>MDFKENPNLRDNWTDAEGYYRVNIGEVLDKRYNVYGYTGQGVFSNVVRARDNARANQEVAVKIIRNNELMQKTGLKELEFLKKLNDADPDDKFHCLRLFRHFYHKQHLCLVFEPLSMNLREVLKKYGKDVGLHIKAVRSYSQQLFL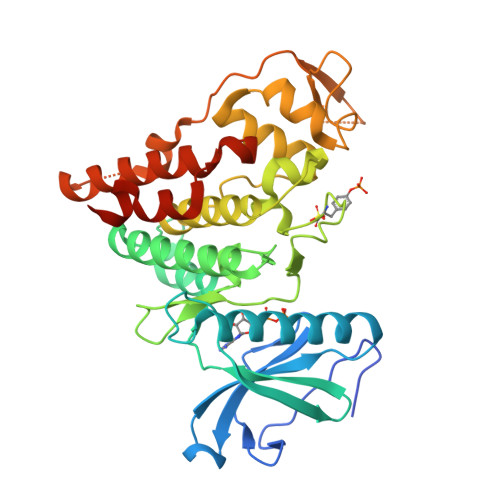ALKLLKRCNILHADIKPDNILVNESKTILKLCDFGSASHVADNDITPYLVSRFYRAPEIIIGKSYDYGIDMWSVGCTLYELYTGKILFPGKTNNHMLKLAMDLKGKMPNKMIRKGVFKDQHFDQNLNFMYIEVDKVTEREKVTVMSTINPTKDLLADLIGCQRLPEDQRKKVHQLKDLLDQILMLDPAKRISINQALQHAFIQEKIHHHHHH[2x]>[2x]MAHHGVSGLVGKLVTQLEVNCDADIFYKIVKHHEEVPNVIPHFFTGVQVTKGDGLVSGCIKEWNYVLEGKAMTAVEETTHADETRTLTHHITEGDAMKDYKKFDVIVETNPKPNGHGSVVTYSIVYEKINEDSPAPFDYLKFFHQNIVDMSAHICSSA

The contiguous latex includes an abundance of related proteins belonging to the pathogenesis-related (PR)10 family known collectively as major latex proteins (MLPs) and representing at least 35% of the total cellular protein content. Members of the pathogenesis-related (PR)10 family, also known as Bet v 1 or major latex proteins (MLPs), belong to the wider ‘StARkin’ lipid-transfer protein (LTP) classification with diverse physiological roles in plants, including sterol trafficking, lipid ‘sensor’ activity, and modulation of transcription factor function. Using a combination of sucrose density-gradient fractionation-coupled proteomics, differential scanning fluorimetry, isothermal titration calorimetry, and X-ray crystallography, we show that the major latex proteins are a family of alkaloid-binding proteins that display altered conformation in the presence of certain ligands. Seven antiparallel β-strands cradle the C-terminal α-helix with the alkaloid binding pocket located in a hydrophobic pocket between the central C-terminal α-helix and the β-sheet.

In the absence of a bound alkaloid, W63 rotates to occupy the hydrophobic binding pocket. Alkaloid binding leads to the ordering of β2 completing the Bet v 1-fold. Alkaloid binding and subsequent ordering of the β2 strand causes C59 to be buried. S-S bonding is potentially a key factor in the ability of opium poppy latex proteins to bind alkaloids and form dense aggregates.>LRVQPEAQAKVDVFREDLCTKTENLLGSYFPKKISELDAFLKEPALNEANLSNLKAPLDI[7x];>[7x]AVNCNEKIVVLLQRLKPEIKDVIEQLNLVTTWLQLQIPRIEDGNNFGVAVQEKVFEL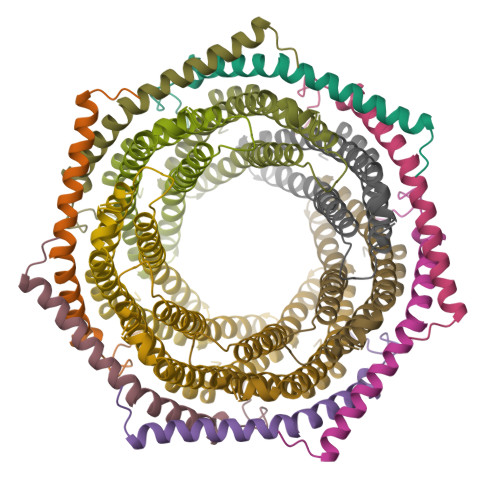MTSLHTKLEGFHTQISKYFSERGDAVTKAAKQPHVGDYRQLVHELDEAEYRDIRLMVMEIRNAYAVLYDIILKNFEKLKKPRG> GSHMSSITKRLYHPKVIEHYTHPRNVGS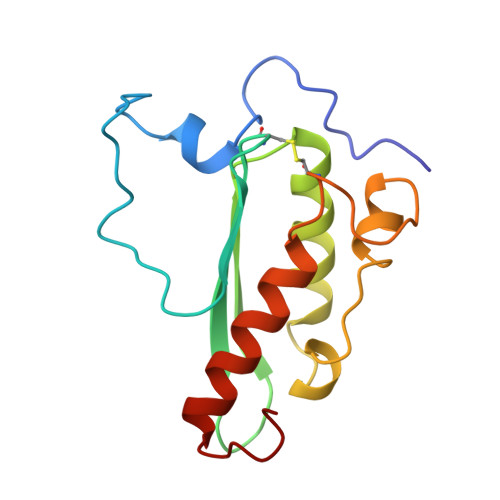LDKKLPNVGTGLVGAPACGDVMRLQIKVNDSTGVIEDVKFKTFGCGSAIASSSYMTELVQGMTLDDAAKIKNTEIAKELSLPPVKLHCSMLAEDAIKAAIKDYKSKRNTPTMLS>[60x]GSGVGHSTGDYNNRTEFIYHGDEVTIICHSTRLVHINMSDREDYIIYETDRGPLFPTTQDLQGRDTLNDSYHAKVETPWKLLHANSWGCWFSPADFQQMITTCRDIAPIQMHQKIENIVIKTVSKTGTGETETTNYNNDLTALLQIAQDNSNLLPWAADNFYIDSVGYVPWRACKLPTYCYHVDTWNTIDINQADTPNQWREIKKGIQWDNIQFTPLETMINIDLLRTGDAWQSGNYTFHTKPTNLAYHWQSQRHTGSCHPTVAPLVERGQGTNIQSVNCWQWGDRNNPSSASTRVSNIHIGYSFPEWQIHYSTGGPVINPGSAFSQAPWGST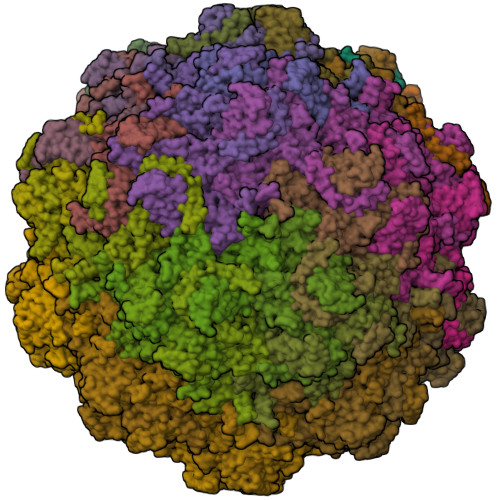TEGTRLTQGASEKAIYDWSHGDDQPGARETWWQNNQHATGQTDWAPKNAHTSELNNNVPAATHFWKNSYHNTFSPFTAVDDHGPQYPWGAIWGKYPDTTHKPMMSAHAPFLLHGPPGQLFVKLAPNYTDTLDNGGITHPRIVTYGTFWWSGKLVFKGKLRTPRQWNTYNLPSLDKRETMKNTVPNEVGHFELPYMPGRCLPNYTL> GSHMGSADEERDHWQQFYFLSKRRRNLLRNPCGEEDLEGWSDVEHGGDGWKVEELPGDNGVEFTQDDSVKKYFASSFEWCRKAQVIDLQAEGYWEELLDTTQPAIVVKDWYSGRTDAGSLYELTVRLLSENEDVLAEFATGQVAVPEDGSWMEISHTFIDYGP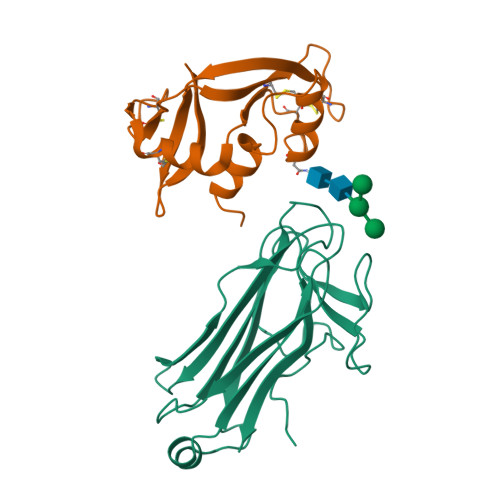GVRFVRFEHGGQDSVYWKGWFGARVTNSSVWVEP;> KETAAAKFERQHMDSSTSAASSSNYCNQMMKSRNLTKDRCKPVNTFVHESLADVQAVCSQKNVACKNGQTNCYQSYSTMSITDCRETGSSKYPNCAYKTTQANKHIIVACEGNPYVPVHFDASV3-(6-{[3-(2,6-dichlorophenyl)-5-(1-methylethyl)isoxazol-4-yl]methoxy}-1-benzothiophen-2-yl)benzoic acid | C28 H21 Cl2 N O4 S | 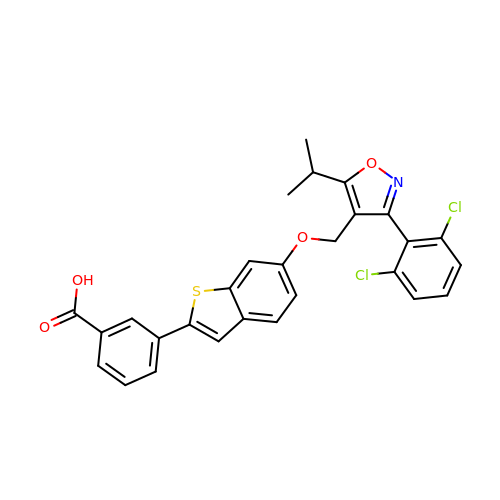WPHVYHBQJIXGIJ-UHFFFAOYSA-N> TKNKDGVLVDEFGLPQ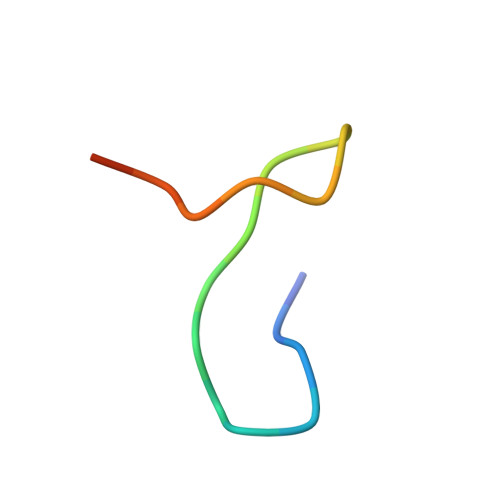IPAS> MSTSWSDRLQNAADMPANMDKHALKKYRREAYHRVFVNRSLAMEKIKCFGFDMDYTLAVYKSPEYESLGFELTVERLVSIGYPQELLSFAYDSTFPTRGLVFDTLYGNLLKVDAYGNLLVCAHGFNFIRGPETREQYPNKFIQRDDTERFYILNTLFNLPETYLLACLVDFFTNCPRYTSCETGFKDGDLFMSYRSMFQDVRDAVDWVHYKGSLKEKTVENLEKYVVKDGKLPLLLSRMKEVGKVFLATNSDYKYTDKIMTYLFDFPHGPKPGSSHRPWQSYFDLILVDARKPLFFGEGTVLRQVDTKTGKLKIGTYTGPLQHGIVYSGGSSDTICDLLGAKGKDILYIGDHIFGDILKSKKRQGWR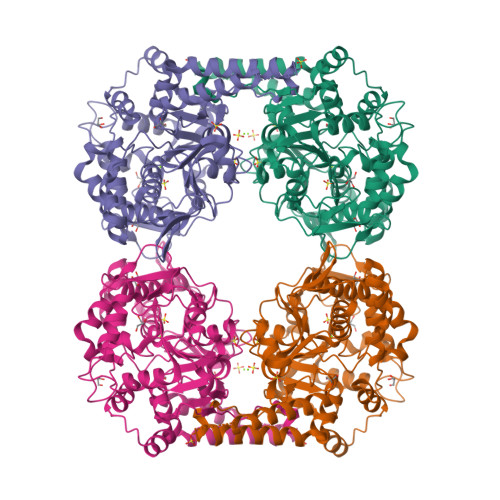TFLVIPELAQELHVWTDKSSLFEELQSLDIFLAELYKHLDSSSNERPDISSIQRRIKKVTHDMDMCYGMMGSLFRSGSRQTLFASQVMRYADLYAASFINLLYYPFSYLFRAAHVLMPHESTVEHTHVDINEMESPLATRNRTSVDFKDTDYKRHQLTRSISEIKPPNLFPLAPQEITHCHDEDDDEEEEEEEE The C-protein C.Esp1396I is a member of a large class of helix-turn-helix proteins that act as transcriptional regulators of gene expression in both prokaryotic and eukaryotic systems. C.Esp1396I finely regulates a bacterial restriction-modification system, providing a delay in endonuclease expression via a concentration-dependent ‘on’ and ‘off’ switch. The C-protein–DNA operator complex consists of two ‘controller’ C-protein dimers (chains A and B, chains C and D) bound to a 35 bp DNA operator sequence (chains E and F). The dsDNA is distorted in the complex, due to binding of protein dimers to each operator site, resulting in minor groove compression (leading to a 50° bend at each binding site) and large major groove expansion at the DNA sequence centre.

Here a model protein–DNA complex C.Esp1396I is employed to investigate specific damage mechanisms for protein and DNA in a biologically relevant complex over a large dose range (2.07–44.63 MGy). To investigate the distribution of specific damage throughout the C.Esp1396I protein–DNA structure with respect to increasing radiation dose, eight successive datasets on the same C.Esp1396I crystal were collected, each exposing the same 100° wedge of the crystal to X-ray radiation. The final model for the first dataset was refined to a resolution of 2.8 Å. In agreement with the original structure, each asymmetric unit contained one tetrameric protein–DNA complex and had a solvent content of 68.7%. At low doses the protein was observed to be susceptible to radiation damage while the DNA was far more resistant, damage only being observed at significantly higher doses. Residues such as Asp, Glu, Met and Ser can be seen to accumulate significant damage (loss of electron density around the Ser side chain –OH) even at the lowest doses.

>[4x]GSHMESFLLSKVSFVIKKIRLEKGMTQEDLAYKSNLDRTYISGIERNSRNLTIKSLELIMKGLEVSDVVFFEMLIKEILKHD Tyrosinases belong to the type 3 copper-containing protein family together with hemocynanins that serve as oxygen carriers, and catechol oxidases that are strict diphenolases34. Tyrosinases hydroxylate monophenols to form ortho-diphenols (monophenolase activity) and subsequently oxidize the o-diphenols to o-quinones (diphenolase activity). The two copper ions in the conserved active site, CuA and CuB, are coordinated by six histidine residues567. In this study, we elucidate the inhibition mechanism of these inhibitors by crystal structure determination of TyrBm with bound KA and HQ in the active site, along with biochemical characterizations, binding constants determination and molecular modeling.

We present here the crystal structure of TyrBm with KA bound in the active site at 2.6 Å resolution. Here, by modifying our protocol for ligand binding in crystal, we have visualized the structure of TyrBm with KA bound in the active site similar to tyrosinase substrates. In the active site, KA is stabilized by π-π interactions with His208 that coordinates CuB, similar to tyrosinase substrates, as presented by Goldfeder et al. and suggested in other studies. The hydroxyl group of KA is oriented towards CuA with a distance of 3.3 Å, while the distance of the carbonyl group to CuA is 5.5 Å. These results are supported by a recent docking study of Lima et al., and contradict a previously proposed inhibition mechanism of KA by copper chelation. However, the two orientations of KA, which are demonstrated by crystallography and in silico simulations, support the mixed inhibition mechanism, which is confirmed by our kinetic experiments. We suggest that when KA is bound strongly in the active site, the binding pocket is not accessible to substrate molecules, subsequently TyrBm is not active. However, when KA is oriented at the entrance of the active site, it restricts substrate entrance and product efflux, consequently, TyrBm cannot reach its maximum velocity.

>KYRVRKNVLHLTDTEKRDFVRTVLILKEKGIYDRYIAWHGAAGKFHTPPGSDRNAAHMSSAFLPWHREYLLRFERDLQSINPEVTLPYWEWETDAQMQDPSQSQIWSADFMGGNGNPIKDFIVDTGPFAAGRWTTIDEQGNPSGGLKRNFGATKEAPTLPTRDDVLNALKITQYDTPPWDMTSQNSFRNQLEGFINGPQLHNRVHRWVGGQMGVVPTAPNDPVFFLHHANVDRIWAVWQIIHRNQNYQPMKNGPFGQNFRDPMYPWNTTPEDVMNHRKLGYVYDIEL[2x]>[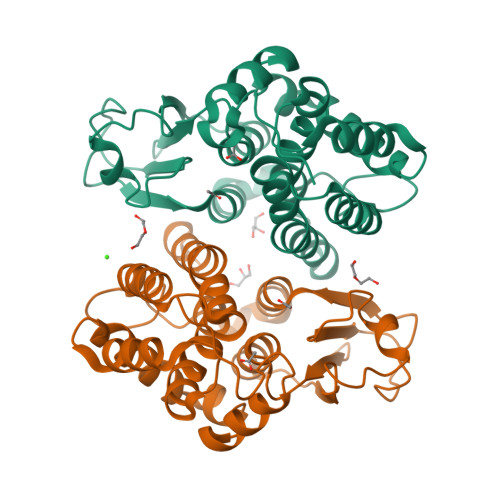2x]MSSTKQITLYTATFSPYAHRVRIALEEAGAEYTTYDVDILRNMPDWFPLVNPLKKIPAMTFGGPEVPPDQPSPESAKIAESLAMLEFIADLFPDAKLLPTDPVLRARARTFMALYENYVNGQFRDVWFLGTPADPLLQALEMLQGALPPDGGFAAGEWSIADAAVIPFLARMFPYLEAGLGLYSKEDGVKMRKAMASERFARIRQYVRDCRARPSFANTWAGDAEQVEAAKTVPMLRVGEHHHHHH> GSEESQAFQRQLTALIGYDVTDVSNVHDDELEFTRRGLVTPRMAEVASRDPKLYAMHPWVTSKPLPEYLWKKIANNCIFIVIHRSTTSQTIKVSPDDTPGAILQSFFTKMAKKKSLMDIPESQSEQDFVLRVCGRDEYLVGETPIKNFQWVRHCLKNGEEIHVVLDTPPDPALDEVRKEEWPLVDDCTGVTGYHEQLTIHGKDHESVFTVSLWDCDRKFRVKIRGIDIPVLPRNTDLTVFVEANIQHGQQVLCQRRTSPKPFTEEVLWNVWLEFSIKIKDLPKGALLNLQIYCGKAPALSSKASAESPSSESKG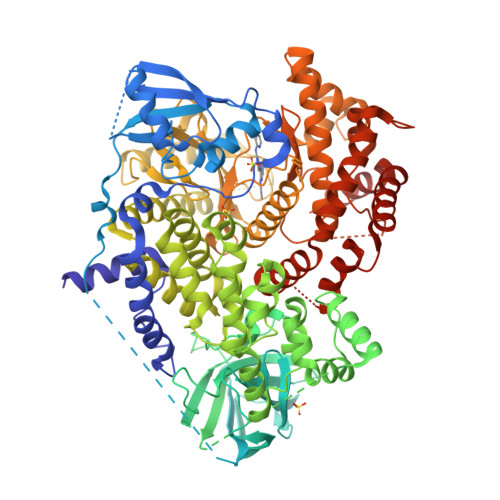KVQLLYYVNLLLIDHRFLLRRGEYVLHMWQISGKGEDQGSFNADKLTSATNPDKENSMSISILLDNYCHPIALPKHQPTPDPEGDRVRAEMPNQLRKQLEAIIATDPLNPLTAEDKELLWHFRYESLKHPKAYPKLFSSVKWGQQEIVAKTYQLLARREVWDQSALDVGLTMQLLDCNFSDENVRAIAVQKLESLEDDDVLHYLLQLVQAVKFEPYHDSALARFLLKRGLRNKRIGHFLFWFLRSEIAQSRHYQQRFAVILEAYLRGCGTAMLHDFTQQVQVIEMLQKVTLDIKSLSAEKYDVSSQVISQLKQKLENLQNSQLPESFRVPYDPGLKAGALAIEKCKVMASKKKPLWLEFKCADPTALSNETIGIIFKHGDDLRQDMLILQILRIMESIWETESLDLCLLPYGCISTGDKIGMIEIVKDATTIAKIQQSTVGNTGAFKDEVLNHWLKEKSPTEEKFQAAVERFVYSCAGYCVATFVLGIGDRHNDNIMITETGNLFHIDFGHILGNYKSFLGINKERVPFVLTPDFLFVMGTSGKKTSPHFQKFQDICVKAYLALRHHTNLLIILFSMMLMTGMPQLTSKEDIEYIRDALTVGKNEEDAKKYFLDQIEVCRDKGWTVQFNWFLHLVLGIKQGEKHSA>[2x]MEPRMESCLAQVLQKDVGKRLQVGQELIDYFSDKQKSADLEHDQTMLDKLVDGLATSWVNSSNYKVVLLGMDILSALVTRLQDRFKAQIGT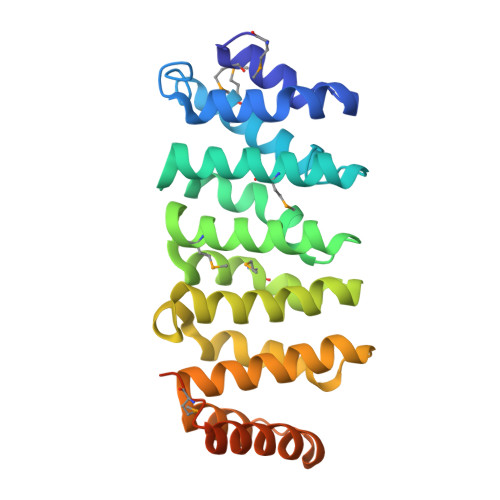VLPSLIDRLGDAKDSVREQDQTLLLKIMDQAANPQYVWDRMLGGFKHKNFRTREGICLCLIATLNASGAQTLTLSKIVPHICNLLGDPNSQVRDAAINSLVEIYRHVGERVRADLSKKGLPQSRLNVIFTKFDEVQKSGNMIQSANDKNFDDEDSVDGNRPSSASS>MGHHHHHHHHLVPRGSMFADLDYDIEEDKLGIPTVPGKVTLQKDAQNLIGISIGGGAQYCPCLYIVQVFDNTPAALDGTVAAGDEITGVNGRSIKGKTKVEVAKMIQEVKGEVTIHYNKLQQSAV[2x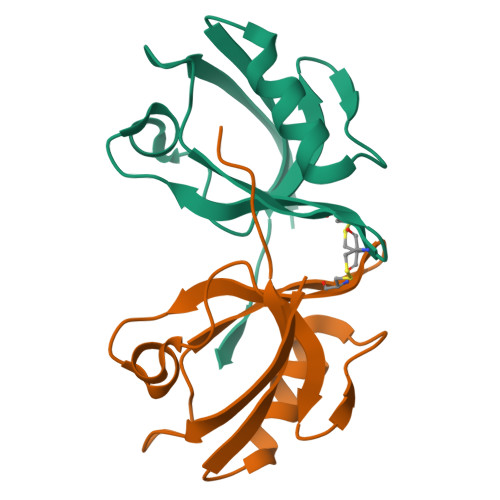]>[2x]MEDMILTEEMQKIMNLIQDDENNVFVTGKAGSGKTTFLKYLIE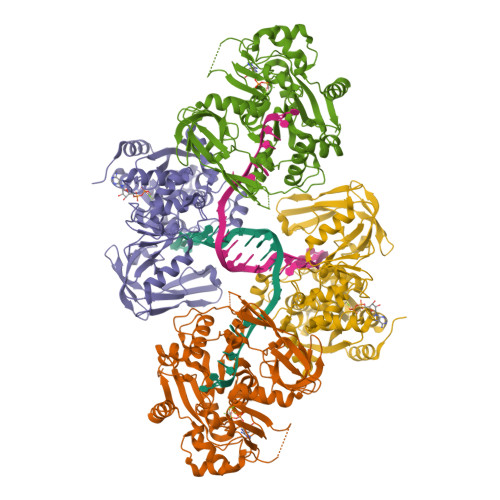KSGKNCIVAAPTGIAAINAGGVTLHSLFGIPFGPITPYDRLENKFSEYKVELLLKMELLIIDEISMVRPDILDTIDRKLRWVYESDEPFGGVQVVMFGDLFQLPPVTKKQEREILSDFYDGFFFFNALVFKRTGFHIVELTKIFRQTEPEFINVLNNIRNYQVTSDELDLLSELKDRKISSSYDNEYIHICTHKADVEKINADKLGEQEIRNYDIVIKDKFPESSIPCDLHLKLRVGARVMSLVNDSLKGYYNGMLGIVTALEDNVITVRMDNGRTIKFERYTWSNTQYTLKDNEIVKEEIGSCTQFPLTLAWAITIHKSQGLTFDKIIIHVSHTFCPGQLYVALSRCRTLEGIVSDAFITKQMIIPEYALIDFERAYKSEGNYYGKRLD> GYQPEKHAVVKSDRGDGRLLSTYAIVHEMLKDTHPQYAYRSGMSAQEFTQWQDGVRAAMVEIMKFPEIKRQPSPVCVKTEKKEGYILEKWEFYPFPKSVSTFLVLKPEHLKGAVPGVLCIPGSGRTKEGLVGEPGICDKLTEDYNNPKVSMALNMVKEGYVAVAVDNAAAGEASDLECYDKGWNYDYDVVSRFLLELGWSWLGYTSYLDMQVLNWMKAQSYIRKDRIVISGFSLGTEPMMVLGVLDKDIYAFVYNDFLCQTQERAVVMTKPDKEN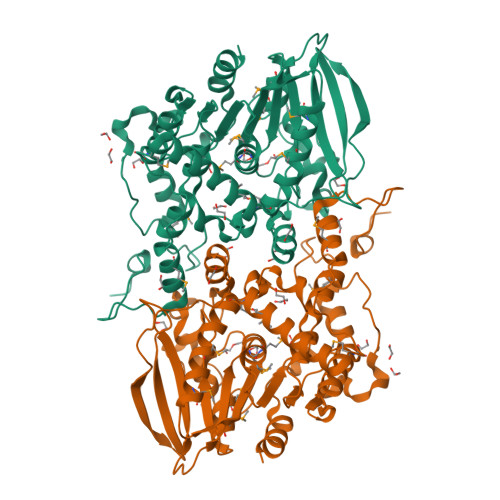RRPFPNSIRHLIPGYWRYFNFPDVVASLAPRPIIFTEGGLDRDFRLVQSAYAASGKPENAEFHHYPKFADKAVRKDVEHLDEGLDSKTYFEAVNVDPPSHYFKNELVIPWLRKVLK Energy-coupling factor (ECF)-type transporters mediate the import of micronutrients, such as folate, cobalamin and pantothenate, in the majority of prokaryotes. A tripartite ATP-hydrolysing motor (ECF module), composed of a membrane-embedded scaffold protein (EcfT) and two cytosolic nucleotide-binding proteins or ATPase subunits (often hetero-dimeric - EcfA and EcfA’), forms a functional core complex with a membrane-embedded substrate-translocating protein (S-component). Structural and biophysical analyses of ECF transporter complexes from three different organisms, with different substrate specificities, and from different laboratories revealed that the core complex and minimal functional unit exists in a 1:1:1:1 subunit stoichiometry. Based on these fragmented structural insights, a model for the transport mechanism has been proposed in which a substrate-free solitary S-component with an outward-facing binding site topples within the membrane upon substrate acquisition, associates with the ECF module, and exposes the binding site to the cytosol, thereby moving the substrate across the membrane.

We then obtained a cryo-EM reconstruction of the nucleotide-free solitary ECF module in lipid nanodiscs at 3.8 Å resolution that shows a vacant docking site for the S-component. The ATPase dimer adopts an open conformation, and the structure of the module is very similar to the conformation observed in full ECF transporter complexes presented above (rmsd: 1.8 Å), as well as to the ECF modules of previously determined structures of the folate-, pantothenate- and cobalamin-specific ECF transporters from L. delbrueckii (rmsd: 1.6–1.8 Å). The main difference is that transmembrane helix 3 and the regions close to the extracellular side of the EcfT subunit in the solitary ECF module are less well resolved. We attribute this to a higher degree of flexibility caused by the absence of any stabilising effect typically exerted by a bound S-component. Notably, in the solitary ECF module, the docking site for the S-component remained structurally intact and unaltered compared to the docking site in the ECF-FolT2 complex. Yet, in contrast to the full complex, it is accessible to the lipid nanodisc environment. Moreover, the docking site is hydrophobic, and, therefore, compatible to interact with the surrounding environment of the lipid nanodisc. In the ATPase open conformation, the lipid nanodisc has a dramatically increased thickness around the empty docking site. The observed thickness of ~50 Å in this area is needed to avoid the exposure of the hydrophobic docking site to the aqueous environment. Moreover, the imposed tension by the convex shape of the coupling helices in the closed conformation may not be energetically favourable and was captured due to the mutations introduced. Thus, the solitary ECF module in the open conformation likely represents an energetically more favourable post-ATP-hydrolysis and relaxed state (Fig. 4–State 3).

> GSDNIISFDHVTFTYPDSPRPALSDLSFAIERGSWTALIGHNGSGKSTVSKLINGLLAPDDLDKSSITVDGVKLGADTVWEVREKVGIVFQNPDNQFVGATVSDDVAFGLENRAVPRPEMLKIVAQAVADVGMADYADSEPSNLSGGQKQRVAIAGILAVKPQVIILDESTSMLDPEGKEQILDLVRKIKEDNNLTVISITHDLEEAAGADQVLVLDDGQLLDQGKPEEIFPKVEMLKRIGLDIPFVYRLKQLLKERGIVLPDEIDDDEKLVQSLWQLNSKM;> MAIKFENVSYVYSPGSPLEAIGLDQLNFSLEEGKFIALVGHTGSGKSTLMQHFNALLKPTSGKIEIAGYTITPETGNKGLKDLRRKVSLAFQFSEAQLFENTVLKDVEYGPRNFGFSEDEAREAALKWLKKVGLKDDLIEHSPFDLSGGQMRRVALAGVLAYEPEIICLDEPAAGLDPMGRLEMMQLFKDYQAAGHTVILVTHNMDDVADYADDVLALEHGRLIKHASPKEVFKDSEWLQKHHLAEPRSARFAAKLEAAGLKLPGQPLTMPELADAIKQSLKGGEHE;> MSKIIIGRYLPGTTFVYRVDPRAKLLTTFYFIIMIFLANNWVSYLVISIFGLAYVFATGLKARVFWDGVKPMIWMIVFTSLLQTFFMAGGKVYWHWWIFTLSSEGLINGLYVFIRFAMIILVSTVMTVTTKPLEIADAMEWMLTPLKLFKVNVGMISLVISIALRFVPTLFDQTVKIMNAQRSRGADFNDGGLVKRAKSVVPMLVPLFIDSLEVALDLSTAMESRGYKGSEGRTRYRILEWSKVDLIPVAYCLLLTILMITTRKH> DKRLRDNHE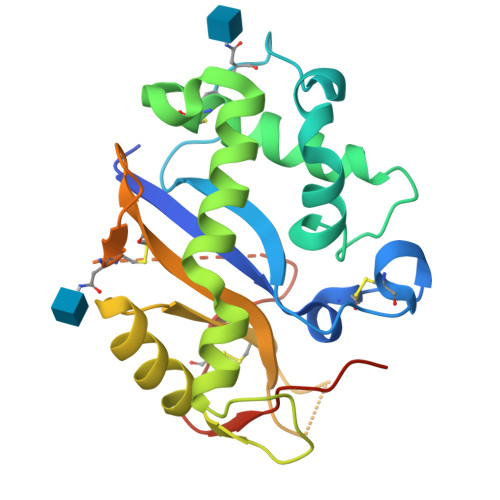WKKLIMVQHWPETVCEKIQNDCRDPPDYWTIHGLWPDKSEGCNRSWPFNLEEIKDLLPEMRAYWPDVIHSFPNRSRFWKHEWEKHGTCAAQVDALNSQKKYFGRSLELYRELDLNSVLLKLGIKPSINYYQVADFKDALARVYGVIPKIQCLPPSQDEEVQTIGQIELCLTKQDQQLQNCTEPGEQPSPKQEVWLANGAAESRGLRVCEDGPVFYPPPKKTKHHHHHHH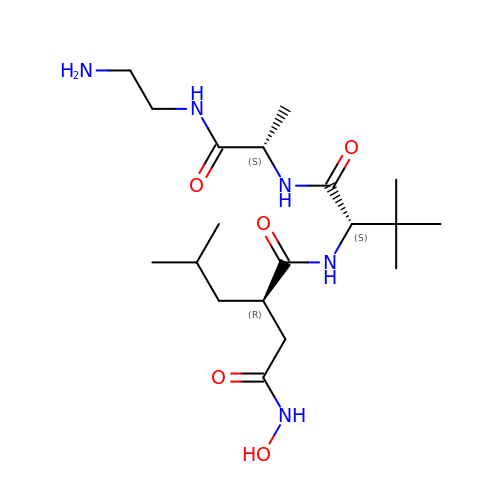N-{(2R)-2-[2-(hydroxyamino)-2-oxoethyl]-4-methylpentanoyl}-3-methyl-L-valyl-N-(2-aminoethyl)-L-alaninamide | C19 H37 N5 O5 | LMIQCBIEAHJAMZ-GZBFAFLISA-N>[2x]GPGGSSMGTLGARRGLEWFLGFYFLSHIPITLLMDLQGVLPRDLYPVELRNLQQWYIEEFKDPLLQTPPAWFKSFLFCELVFQL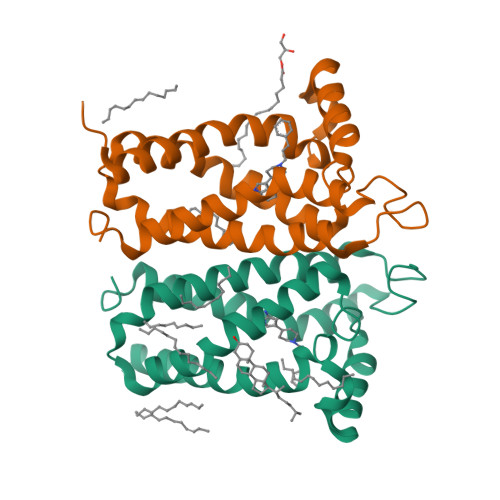PFFPIAAYAFFKGGCKWIRTPAIIYSVHTMTTLIPILSTLLLDDFSKASHFRGQGPKTFQERLFLISVYIPYFLIPLILLLFMVRNPYYK>[2x]GSHMKEVSEHCSHMIGNGHLKVLQQLID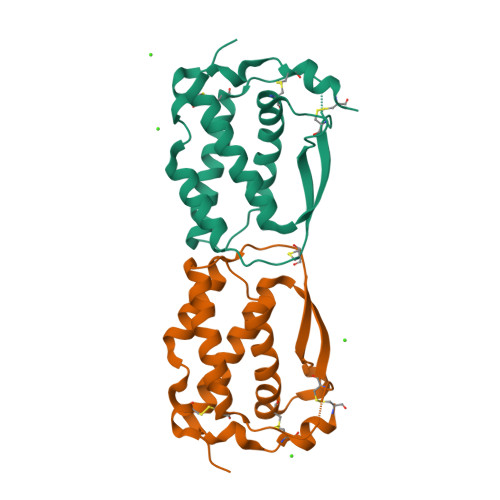SQMETSCQIAFEFVDQEQLDDPVCYLKKAFFLVQDIIDETMRFKDNTPNANATERLQELSNNLNSCFTKDYEEQNKACVRTFHETPLQLLEKIKNFFNETKNLLEKDWNIFTKNCNNSFAKCSSR> GSHMSNISLIVGLGNPGSEYAQTRHNAGFWFVEQLADKYGITLKNDPKFHGISGRGNIEGHDVRLLLPMTYMNKSGQSVVPFSKFYQIAPEAILIAHDELDMNPGVIRLKTGGGHGGHNGLRDIVPH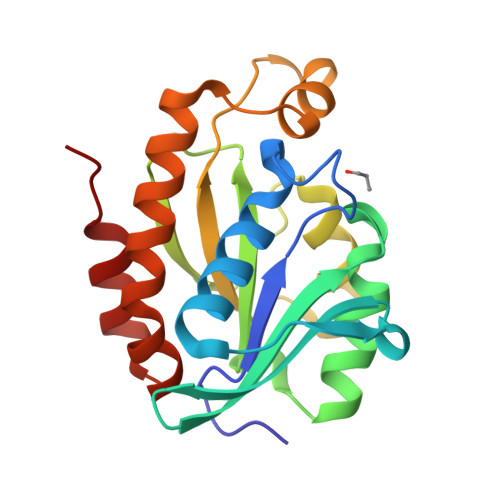IGPNFHRLRIGIGHPGSKERVSGHVLGKAPSNEQSLMDGAIDHALSKVKLLVQGQVPQAMNQINAYKPA(1-HYDROXY-1-PHOSPHONO-2-[1,1';3',1'']TERPHENYL-3-YL-ETHYL)-PHOSPHONIC ACID | 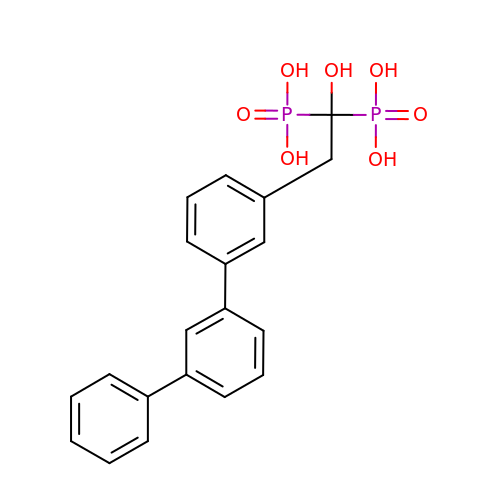C20 H20 O7 P2 | YXQQNSYZOQHKHD-UHFFFAOYSA-N> LEEKKVCQGTSNKLTQLGTFEDHFLSLQRMFNNCEVVLGNLEITYVQRNYDLSFLKTIQEVAGYVLIALNTVERIPLENLQIIRGNMYYENSYALAVLSNYDANKTGLKELPMRNLQEILHGAVRFSNNPALCNVESIQWRDIVSSDFLSNMSMDFQNHLGSCQKCDPSCPNGSCWGAGEENCQKLTKIICAQQCSGRCRGKSPSDCCHNQCAAGCTGPRESDCLVCRKFRDEATCKDTCPPLMLYNPTTYQMDVNPEGKYSFGATCVKKCPRNYVVTDHGSCVRACGA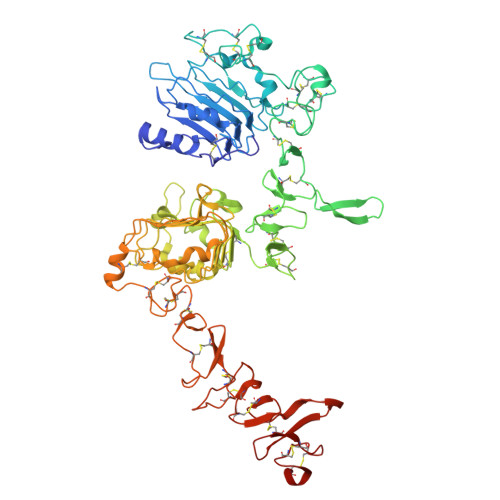DSYEMEEDGVRKCKKCEGPCRKVCNGIGIGEFKDSLSINATNIKHFKNCTSISGDLHILPVAFRGDSFTHTPPLDPQELDILKTVKEITGFLLIQAWPENRTDLHAFENLEIIRGRTKQHGQFSLAVVSLNITSLGLRSLKEISDGDVIISGNKNLCYANTINWKKLFGTSGQKTKIISNRGENSCKATGQVCHALCSPEGCWGPEPRDCVSCRNVSRGRECVDKCKLLEGEPREFVENSECIQCHPECLPQAMNITCTGRGPDNCIQCAHYIDGPHCVKTCPAGVMGENNTLVWKYADAGHVCHLCHPNCTYGCTGPGLEGCPT> PAKSAPA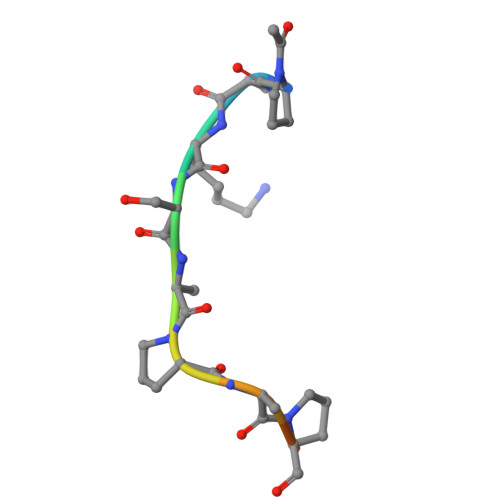PKKG> AGCGAACGTGGATTTTGTCCGACATCGGCAAGCTCCCTTTTTCGACTATT;> CCGATGTCGGACTTTTACACGATCTTCGCCTGCTGGGTTTTGGGAGCTTG;> CGAAGATCGTGTTTTTCCACAGTTGATTGCCCTTCACTTTTCCCAGCAGG;> AATCAACTGTGGTTTTTCTCACTGGTGATTAGAATGCTTTTGTGAAGGGC;> TCACCAGTGAGATTTTTGTCGTACCAGGTGCATGGATTTTTGCATTCTAA;> CCTGGTACGACATTTTTCCACGTTCGCTAATAGTCGATTTTATCCATGCA

We used cryo-EM to investigate the structure of 6HB. This DNA nanoarchitecture is composed of six DNA duplexes assembled from six oligonucleotides. Each duplex folds from two DNA strands which connect to two neighbouring duplexes via interduplex loops. Each duplex features a single-stranded nick region in the barrel midsection. The elongated 6HB structure has a nominal height of ~90 Å with nominal outer and inner channel widths of 50 and 18 Å, respectively.

The particles were sorted into conformational groups, and the five most populated structures were refined during structural analysis. The structures of each group were, on average, resolved at 8 Å, enabling tracing of the six DNA duplex strands in different conformations, while the most flexible poly-thymidine loops were of lower resolution. All five populations deviated from the ideal, designed 6HB structure and adopted a range of structural conformers. For example, the symmetrical hexagonal arrangement of six duplexes was not found in the structures. Instead, the five classes are shorter and wider with a class average of 67.0 ± 0.4 × 71.8 ± 4.0 Å, respectively. Our cryo-EM analysis indicated that the five structural classes feature a bloated cylindrically shaped lumen with a wider centre. The central region of the lumen has an average of 34.0 ± 6.9 Å ranging from 20.7 Å in Class 2 to 40.6 Å in Class 4.3-[[4-(4-ethanoyl-3,5-dimethyl-1~{H}-pyrrol-2-yl)-1,3-thiazol-2-yl]methyl]imidazolidine-2,4-dione 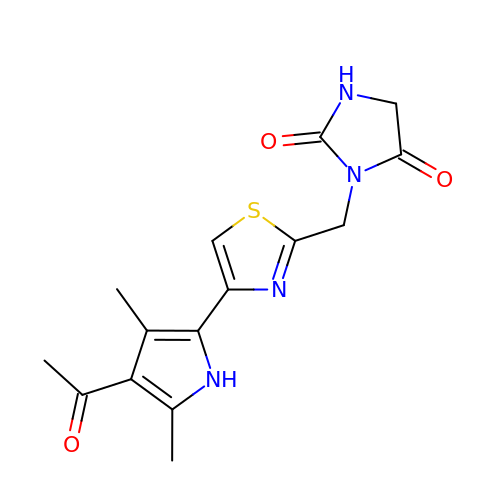| C15 H16 N4 O3 S | XGIZTMPAAINKGM-UHFFFAOYSA-N5-{[4-{[2-(pyrrolidin-1-ylsulfonyl)benzyl]amino}-5-(trifluoromethyl)pyrimidin-2-yl]amino}-1,3-dihydro-2H-indol-2-one 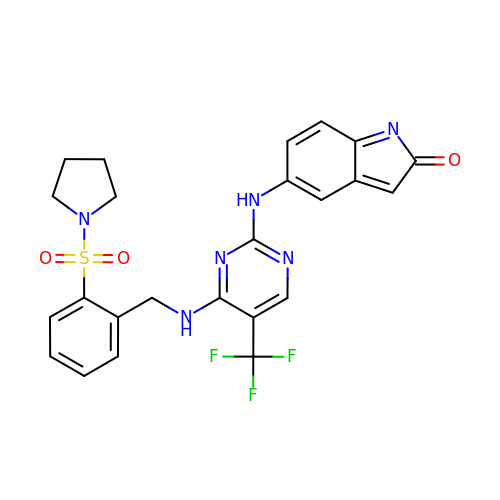| C24 H21 F3 N6 O3 S | TWFBJYGVNVQOCW-UHFFFAOYSA-N[1-[2-[3-[[(2~{R})-4-[[[(2~{R},3~{S},4~{R},5~{R})-5-(6-aminopurin-9-yl)-4-oxidanyl-3-phosphonooxy-oxolan-2-yl]methoxy-oxidanyl-phosphoryl]oxy-oxidanyl-phosphoryl]oxy-3,3-dimethyl-2-oxidanyl-butanoyl]amino]propanoylamino]ethylsulfanyl]-1-oxidanylidene-propan-2-ylidene]-bis(oxidanidyl)azanium | C24 H38 N8 O19 P3 S | 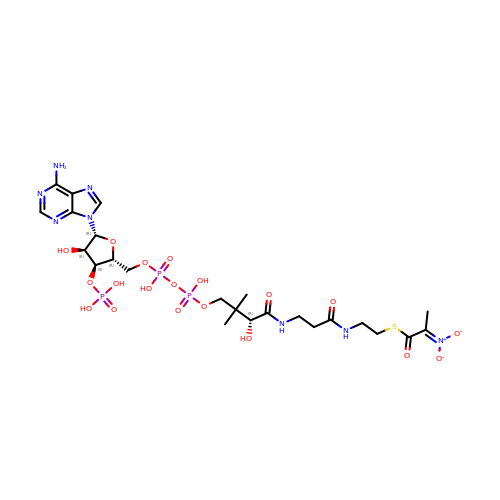BLWVPDVKNPMTPY-ZSJPKINUSA-N>[4x]MSFTIQSAQSIFPGTLVADIVPTVVESFSQLNAEDQLALLWFAYTEMGRSITVAAPGAANMILAQGLLEQIKQMPFEAQTQVMYDLANRADTPL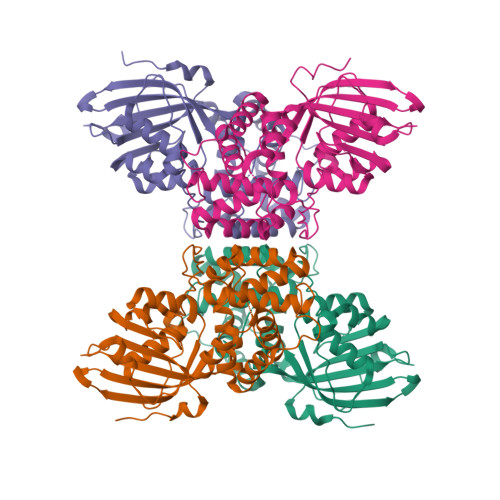CRSYASFTVNIKLGFWYQLGEWMAQGIVAPIPEGYKLSPKAADVLQAIRNADSGQQITILRNTVISMGFDPNAPGSYKKVTEPVSPPTAPAFRTKVTIEGINNATVLGYINNMNANDFDAAVALFRSEGALQPPFERPIVGQDAIRAYMREECQGLKMIPERGISEPVEDGYTQVKVTGKVQTPWFGASVGMNIAWRFLIDPQGKIFFVAIDLLASPKELLNLVRKHHHHHH>MDENAKEPENALDKLFSSEQQASILHVLNTASTKELEAFRLLRGRRSINIVEHRENFGPFQNLESLMNVPLFKYKSTVQVCNSILCPKTGREKRKSPENRFLRKLLKPDIERERLKAVNSIISIVFGTRRIAWAHLDRKLTVLDWQQSDRWSLMRGIYSSSVYLEEISSIISKMPKADFYVLEKTGLSIQNSSLFPILLHFHIMEAMLYALLNKTFAQDGQHQVLSMNRNAVGKHFELMIGDSRT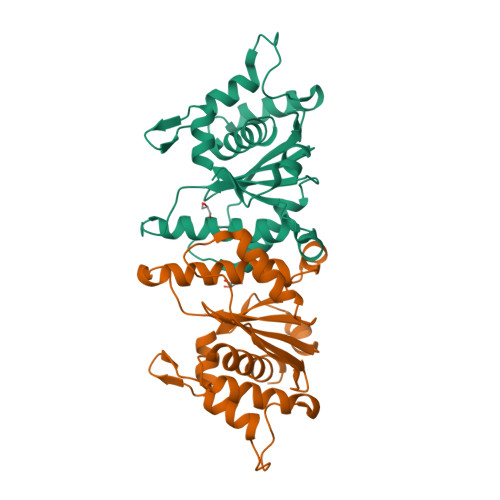SGKELVKQFLFDSILKADPRVFFPSDKIVHYRQMFLSTELQRVEELYDSLLQAIAFYELAVFDSQPLEHHHHHH[4x]N-acetyl-S-({(2R,3S,4R)-3-hydroxy-2-[(1S)-1-hydroxy-2-methylpropyl]-4-methyl-5-oxopyrrolidin-2-yl}carbonyl)cysteine | C15 H24 N2 O7 S | 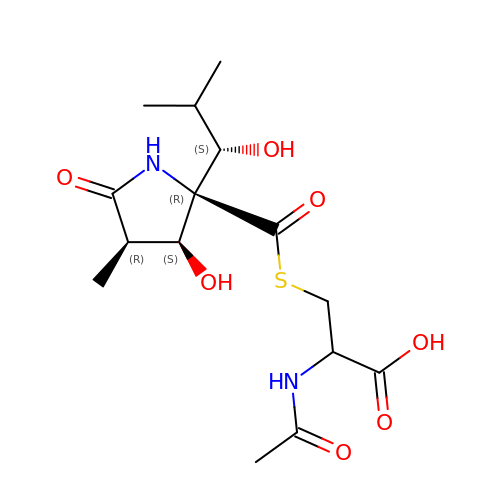DAQAKHDKYAWHCG-MJZHQVMOSA-N> SHMAATAAEAVASGSGEPREEAGALGPAWDESQLRSYSFPTRPIPRLSQSDPRAEELIENEEPVVLTDTNLVYPALKWDLEYLQENIGNGDFSVYSASTHKFLYYDEKKMANFQ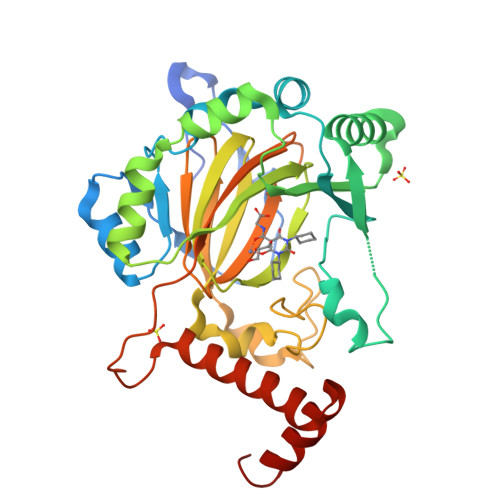NFKPRSNREEMKFHEFVEKLQDIQQRGGEERLYLQQTLNDTVGRKIVMDFLGFNWNWINKQQGKRGWGQLTSNLLLIGMEGNVTPAHYDEQQNFFAQIKGYKRCILFPPDQFECLYPYPVHHPCDRQSQVDFDNPDYERFPNFQNVVGYETVVGPGDVLYIPMYWWHHIESLLNGGITITVNFWYKGAPTPKRIEYPLKAHQKVAIMRNIEKMLGEALGNPQEVGPLLNTMIKGRYN> DYKDDDDAMGRSHTITMTTTSVSSWPYSSHRMRFITNHSDQPPQNFSATPNVTTCPMDEKLLSTVLTTSYSVIFIVGLVGNIIALYVFLGIHRKRNSIQIYLLNVAIADLLLIFCLPFRIMYHINQNKWTLGVILCKVVGTLFYMNMYISIILLGFISLDRYIKINRSIQQRKAITTKQSIYVCCIVWMLALGGFLTMIILTLKKGGHNSTMCFHYRDKHNAKGEAIFNFILVVMFWLIFLLIILSYIKIGKNLLRISKRRSKFPNSGKYATTARNSFIVLIIFTICFVPYHAFRFIYISSQLNVSSCYWKEIVHKTNEIMLVLSSFNSCLDPVMYFLMSSNIRKIMCQLLFRRFQGEPSRSESTSEFKPGYSLHDTSVAVKIQSSSKSTENLYFQ

GPR34 is a recently identified G-protein coupled receptor, which has an immunomodulatory role and recognizes lysophosphatidylserine (LysoPS) as a putative ligand. Here, we report two cryo-electron microscopy (cryo-EM) structures of human GPR34-Gi complex bound to an sn-3 LysoPS derivative and the potent M1 agonist. GPR34 adopts the canonical GPCR topology of a heptahelical transmembrane bundle (7TM), with an extracellular N-terminus, three extracellular loops (ECLs), three intracellular loops (ICLs), and a short amphipathic helix 8 (H8) oriented parallel to the membrane. The ligand-binding pocket of GPR34 extends from the centre of ECL2 to the middle of TM4–5, forming an ~25-Å cleft that is laterally open toward the membrane.

M1 is an analogue of S3E-LysoPS, in which the fragile oleic acid is substituted with a more metabolically stable aromatic fatty acid surrogate (i.e., three tandemly linked phenyl groups, with two ether bonds). Local refinement with the mask of the receptor improved local resolution of the extracellular half of the receptor, and the resulting cryo-EM maps allowed modelling of the entire complexes, including agonists. The overall structure of the M1-bound receptor superimposes well on the S3E-LysoPS-bound structure, with a root-mean-square deviation (RMSD) of 0.73 Å. M1 binds to the hydrophilic and hydrophobic pockets in a pose similar to that of S3E-LysoPS, and the head groups of M1 and S3E-LysoPS form comparable interactions with the hydrophilic pocket. Compared with the S3E-LysoPS-bound form, the extracellular portion of TM4 is displaced outwardly by 2.6 Å, due to key differences in the hydrophobic pockets. However, within the hydrophobic pocket, F2195.39A mutation increased the potency of M1, suggesting that its bulkiness is not essential for M1 binding. In contrast, L2235.43A mutation reduces potency by 10-fold, suggesting that the L-shaped hydrophobic constriction formed by L2235.43 provides the necessary environment for binding M1, but not S3E-LysoPS. Notably, the ligand RMSD (Root Mean Square Deviation) with respect to protein (the same below), illustrating the average change in displacement of ligand for a particular frame with respect to a reference frame (initial frame), is smaller in the M1-bound structure than the S3E-LysoPS-bound structure during the 1-µs MD, indicating that the binding of M1 is more stable than that of S3E-LysoPS. Critically, the metabolically stable agonist M1 nicely fits into the L-shaped hydrophobic pocket in the TM4–5 gap, forming quite stable hydrophilic interactions with the receptor.>GSHMGQGGSNPKFENIAEGLRALLARSHVERTTDEGTWVAGVFVYGGSKTSLYNLRRGTALAIPQCRLTPLSRLPFGMAPGPGPQPGPLRESIVCYFMVFLQTHIFAEVLKDAIKDLVMTKPAPTCNIRVTVCSFDDGVDLP[2x]

Critical for maintaining viral episomes are the homologous Epstein–Barr nuclear antigen 1 (EBNA1) and KSHV latency-associated nuclear antigen (LANA). EBNA1 and LANA bind to specific genetic elements on the viral episome, where they recruit cellular replication machinery to initiate DNA replication, regulate viral gene expression, and tether viral genomes to host chromosomes during mitotic segregation. The DNA-binding domains of EBNA1 and LANA share a similar overall backbone architecture with other viral proteins like human herpesvirus 6A (HHV-6A) immediate early protein 2 (IE2) and human papillomavirus (HPV) E2, but no other human proteins. The stable dimeric core of antiparallel β sheets is surrounded by three critical α-helices that mediate important contacts with the DNA.

We determined the high-resolution crystal structure of one fragment bound to EBNA1. We soaked the fragment AC37287 into preformed crystals of EBNA1 (468–607). The crystal of AC37287 diffracted to 1.3 Ångstroms and was solved by isomorphous replacement. The aliphatic portion of AC37287 binds into a deep hydrophobic pocket made up of the hydrophobic residues I481, L520, L582, V483 and I593. The lactone is sandwiched between residues N519 and T590 within the range of a hydrogen bond of N519. This molecule binds in a region that is important for DNA binding. Superposition of the crystal structures of both EBNA1 bound to AC37287 and to DNA shows that AC37287 binds to a region that sterically clashes with the phosphate backbone of DNA. We identified a coumarin molecule, AC37287, that binds in this pocket of EBNA1 with the potential to inhibit DNA binding. This pocket is made up of a core of hydrophobic residues—Ile481, Leu485, Leu520 and Leu582—surrounded by the polar residues Asn519 and Thr590, which make hydrogen bonding contacts with a DNA phosphate.>[2x]MNLKDKILGVAKELFIKNGYNAT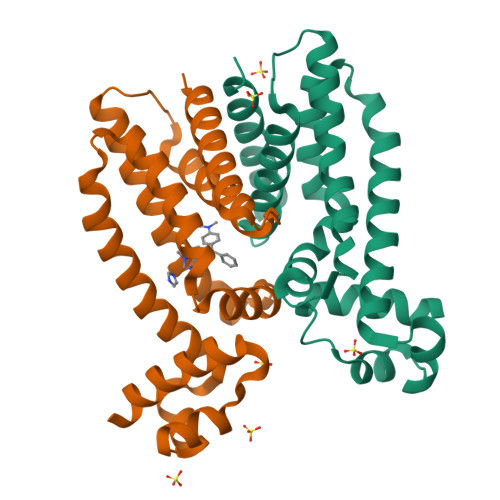TTGEIVKLSESSKGNLYYHFKTKENLFLEILNIEESKWQEQWKKEQIKAKTNREKFYLYNELSLTTQYYYPLQNAIIEFYTEYYKTNSINEKMNKLENKYIDAYHVIFKEGNLNGEWSINDVNAVSKIAANAVNGIVTFTHEQNINERIKLMNKFSQIFLNGLSKHHHHHH> MLDLFADAEPWQEPLAAGAVILRRFAFNAAEQLIRDINDVASQSPFRQMVTPGGYTMSVAMTNCGH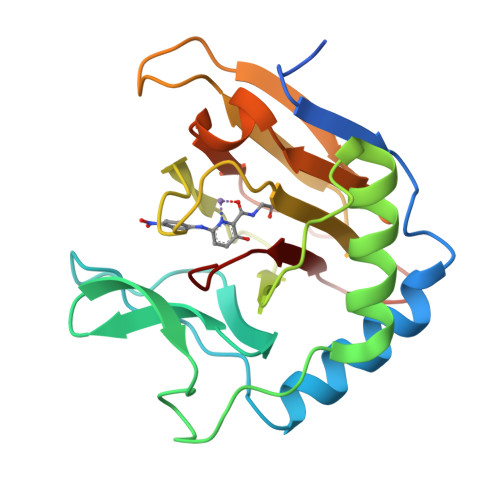LGWTTHRQGYLYSPIDPQTNKPWPAMPQSFHNLCQRAATAAGYPDFQPDACLINRYAPGAKLSLHQDKDEPDLRAPIVSVSLGLPAIFQFGGLKRNDPLKRLLLEHGDVVVWGGESRLFYHGIQPLKAGFHPLTIDCRYNLTFRQAGKKE>SLPMQHVHTSPVRDYRNRCARREGETVFQVVVEETDLRVTALAELATPMAAYVGELRAQLKVWMEFQPAFRHSLVPVEVPEGAPEVVRRMAHGARLVGVGPFAAVAGTIAQMVAERFVDVSPELIVENGGDLYLYSERDRVVGILPDPASGDMVGILVRAGTAPVSLCGSSARIGHSLSLGDGD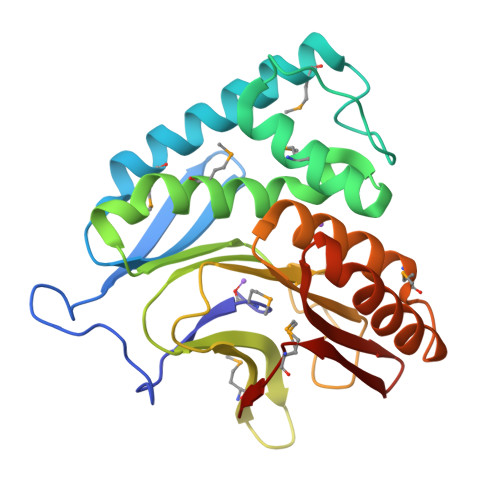LAVVRARDASLADAAATAFGNMLRRADDVAAVTERAAQLASIGIEGVYAQCGGRIGIWGDMELAVA[2x]>[2x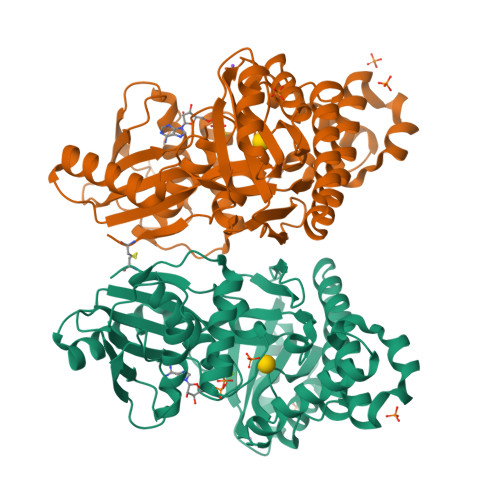]MAALRQPQVAELLAEARRAFREEFGAEPELAVSAPGRVNLIGEHTDYNQGLVLPMALELMTVLVGSPRKDGLVSLLTTSEGADEPQRLQFPLPTAQRSLEPGTPRWANYVKGVIQYYPAAPLPGFSAVVVSSVPLGGGLSSSASLEVATYTFLQQLCPDSGTIAARAQVCQQAEHSFAGMPCGIMDQFISLMGQKGHALLIDCRSLETSLVPLSDPKLAVLITNSNVRHSLASSEYPVRRRQCEEVARALGAASLREVQLEELEAARDLVSKEGFRRARHVVGEIRRTAQAAAALRRGDYRAFGRLMVESHRSLRDDYEVSCPELDQLVEAALAVPGVYGSRMTGGGFGGCTVTLLEASAAPHAMRHIQEHYGGTATFYLSQAADGAKVLCL 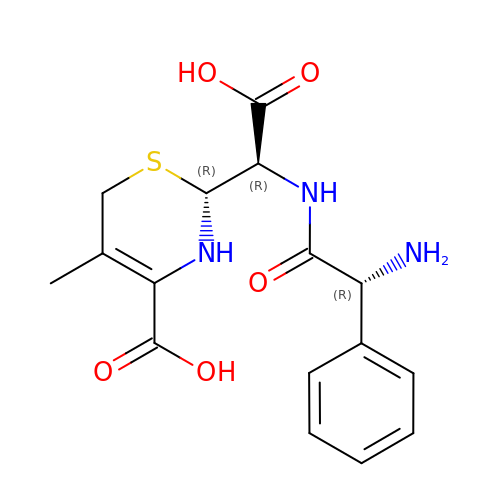(R)-2-((R)-((R)-2-amino-2-phenylacetamido)(carboxy)methyl)-5-methyl-3,6-dihydro-2H-1,3-thiazine-4-carboxylic acid | C16 H19 N3 O5 S | MSGWVKZSYIMFHD-SCDSUCTJSA-N(1R,3R,7E,17beta)-17-[(2R,3S)-3-butyl-5-ethyl-5-hydroxyheptan-2-yl]-2-methylidene-9,10-secoestra-5,7-diene-1,3-diol | C32 H54 O3 | 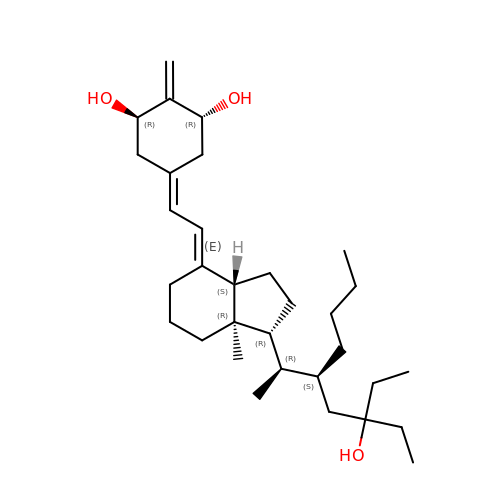OILLQCLQUXHGBN-PWPPSVFISA-N> V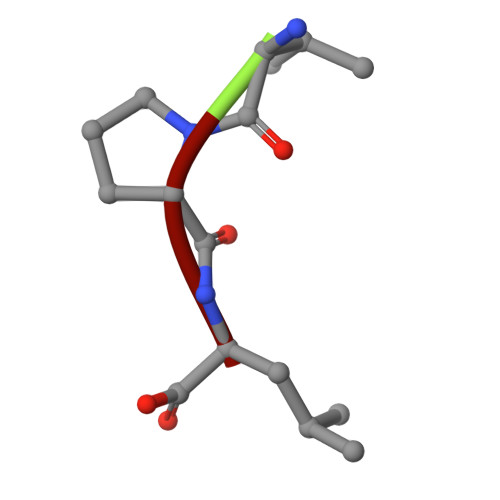PL>[3x]MSISISYSTTYSGWTVADYLADWSAYFGDVNHRPGQVVDGSNTGGFNPGPFDGSQYALKSTASDAAFIAGGDLHYTLFSN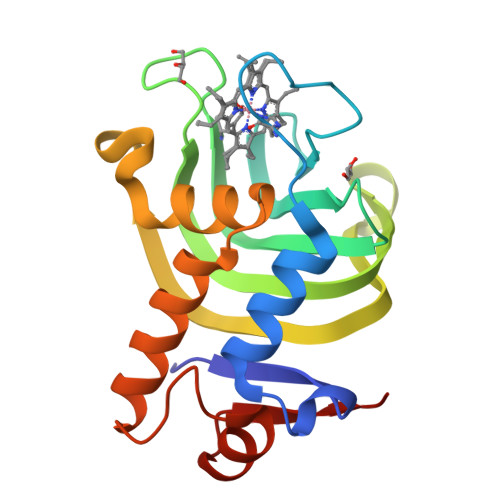PSHTLWGKLDSIALGDTLTGGASSGGYALDSQEVSFSNLGLDSPIAQGRDGTVHKVVYGLMSGDSSALQGQIDALLKAVDPSLSINSTFDQLAAAGVAHATPAA>[4x]MSSLCLQR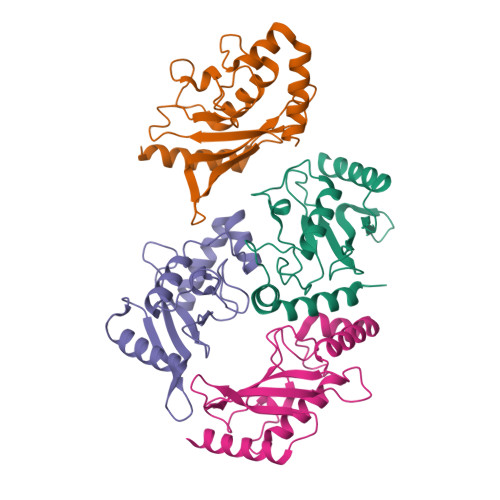LQEERKKWRKDHPFGFYAKPVKKADGSMDLQKWEAGIPGKEGTNWAGGVYPITVEYPNEYPSKPPKVKFPAGFYHPNVYPSGTICLSILNEDQDWRPAITLKQIVLGVQDLLDSPNPNSPAQEPAWRSFSRNKAEYDKKVLLQAKQYSK> TLEPEGAPYWTNTEKMEKRLHAVPAANTVKFRCPAGGNPMPTMRWLK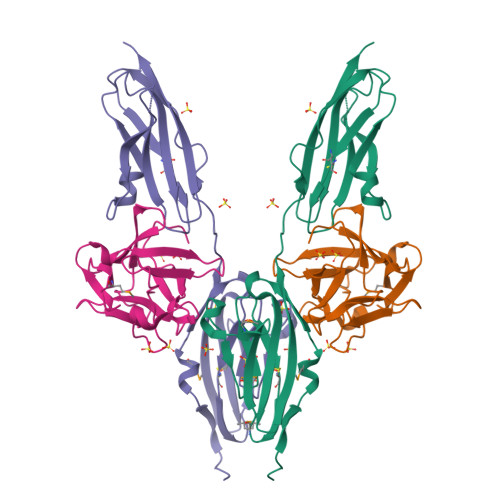NGKEFKQEHRIGGYKVRNQHWSLIMESVVPSDKGNYTCVVENEYGSINHTYHLDVVERSPHRPILQAGLPANASTVVGGDVEFVCKVYSDAQPHIQWIKHVEKNGSKYGPDGLPYLKVLKAAGVNTTDKEIEVLYIRNVTFEDAGEYTCLAGNSIGISFHSAWLTVLPA;> GNYKKPKLLYCSNGGHFLRILPDGTVDGTRDRSDQHIQLQLSAESVGEVYIKSTETGQYLAMDTDGLLYGSQTPNEECLFLERLEENHYNTYISKKHAEKNWFVGLKKNGSCKRGPRTHYGQKAILFLPLPVSSD> MSGSLSRGNGGKKVLNKNQLLKRNRIRNARSIRAEAVAASSTKTGTPSDLSESGSKLNVDQFISSRQFEVKQLQLAMHNSKAASSTRIFQALPRKLRRRTASHNVRRIPKRMRNRALREMRKSDQQDVLKGSSASSRKAHGLNAKQLYKARMSIKLLRLASKSTSMKLSMPPEVTSSNCHVRQKIKTLKRMIKESSTANPNIKLLNNRMGSYDCTGVNELAPIPKGRVKYTKRQKHFAWLPTHIWNAKRSHMMKRWGYQMVWAPTQKCFKLTHRLGGDTCSSDGALCMDSSYIGTIIVKDKSNDSEGDFLKSIIGKLTAERANLRKYREGQVLFQGLIYSFNEENGEDSTKPLGPCDVFWVQKDTAIIRLHPSIYTQVFNILLQHKEKLTVQDCRYSLASVTLKGAKALESLASCLRSTEYSKSFEQFKMVSMITDHNALPQRCTFAFEAIDPRHLAAPKKLNDSQRKTVNSDDILSLHENYPQDEINAVFNELCDPESRTQSYNNQNTLKEISARRYKLLTATPNSINKTTVPFKESDDPSIPLVIIRRLKTRDWIVVLPWFWLLPLWHLLNRIPRMYHIGLRQFQQIQYENKQLYFPDDYPFTQLGYIENSFYKKEASKTKWDRKPMGKRINFEKIKDIHNTKLPAYSGEIGDFFSSDWRFLQILRNGIDYLQRNDKTLELMDSKKTGQFNAQGVRDINCVNDVLEFCKDYEAKTKAMSLSIEENIPVALCKNRKCQFRTPDSISVNSSSFSLTFFPRCIIAVSCTLLERGHPKDNARIYQVPEKDLEHWLQLAKGVYRPNGRKDHDLKIPLPEVHDLIGFITSGTYHLNCGNGMGIGFIDHHAAIRQPTRYVLIRNVGTNTYRLGEWSKISV;> MSGSLKSLDKKIAKRRQVYKPVLDNPFTNEAHMWPRVHDQPLIWQLLQSSIINKLIHIQSKENYPWELYTDFNEIVQYLSGAHGNSDPVCLFVCNKDPDVPLVLLQQIPLLCYMAPMTVKLVQLPKSAMDTFKSVSKYGMLLLRCDDRVDKKFVSQIQKNVDLLQFPWLNAIKYRPTSVKLLKTTVPIVSKKRQK;> MDRTQTFIKDCLFTKCLEDPEKPFNENRFQDTLLLLPTDGGLTSRLQRQQRKSKLNLDNLQKVSQLESADKQLEKRDYQRINKNSKIALREYINNCKKNTKKCLKLAYENKITDKEDLLHYIEEKHPTIYESLPQYVDFVPMYKELWINYIKELLNITKNLKTFNGSLALLKLSMADYNGALLRVTKSKNKTLIGLQGIVIWDSQKFFIMIVKGNIIDEIKCIPKKGTVFQFEIPISDDDDSALRYSILGDRFKYRSVDRAGRKFKSRRCDDMLYYIQN;> MVRLKSRYILFEIIFPPTDTNVEESVSKADILLSHHRASPADVSIKSILQEIRRSLSLNLGDYGSAKCNSLLQLKYFSNKTSTGIIRCHREDCDLVIMALMLMSKIGDVDGLIVNPVKVSGTIKKIEQFAMRRNSKILNIIKCSQSSHLSDNDFIINDFKKIGRENENENEDD;> MINGVYYNEISRDLDISSSTQCLRFLKETVIPSLANNGNNSTSIQYHGISKNDNIKKSVNKLDKQINMADRSLGLQQVVCIFSYGPHIQKMLSILEIFKKGYIKNNKKIYQWNKLTSFDIKREGRNELQEERLKVPILVTLVSDSEIIDLNLHSFTKQ;> MALKKNTHNKSTKRVTKHPSLKTLTHKQIHTTIFVKSTTPYVSALKRINKFLDSVHKQGSSYVAVLGMGKAVEKTLALGCHFQDQKNKKIEVYTKTIEVLDEVITEGQADIDMESDVEDDDKETQLKKRAVSGVELRIYV;> MGKKTFREWQYFKLSITSFDQDVDDAHAIDQMTWRQWLNNALKRSYGIFGEGVEYSFLHVDDKLAYIRVNHADKDTFSSSISTYISTDELVGSPLTVSILQESSSLRLLEVTDDDRLWLKKVMEEEEQDCKCI;>MLVDLNVPWPQNSYADKVTSQAVNNLIKTLSTLHMLGYTHIAINFTVNHSEKFPNDVKLLNPIDIKRRFGELMDRTGLKLYSRITLIIDDPSKGQSLSKISQAFDIVAALPISEKGLTLSTTNLDIDLLTFQYGSRLPTFLKHKSICSCVNRGVKLEIVYGYALRDVQARRQFVSNVRSVIRSSRSRGIVIGSGAMSPLECRNILGVTSLIKNLGLPSDRCSKAMGDLASLVLLNGRLRNKSHKQTIVTGGGSGNGDDVVNDVQGIDDVQTIKVVKRSMDAEQLGHASKRHKP[2x];> MNKDQAEKYQERSLRQKYNLLHVLPTLNSRALSGLYYKNFHNSVKRYQIMLPEQLKSGKFCSHCGCVYVPNFNASLQLTTNTEQGDSDELGGESMEGPKKCIQVNCLNCEKSKLFEWKSEFVVPTFGQDVSPMINSTSSGKVSYAVKKPQKSKTSTGKERSKKRKLNSLTNLLSKRNQEKKMEKKKSSSLSLESFMK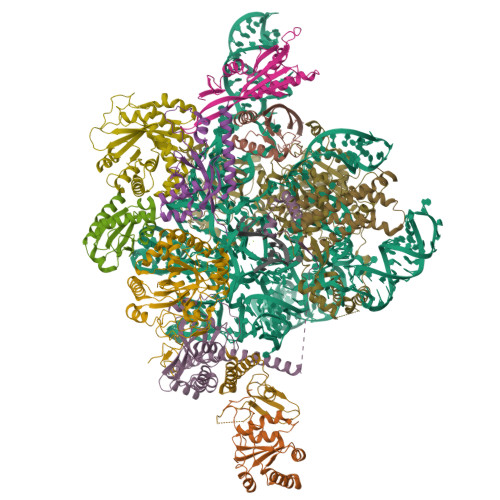S;> MDEMDNVIRSLEQEYRLILLLNHRNKNQHRAASWYGSFNEMKRNCGQIITLFSSRRLQAKRLKDVEWVKLHRLLQRALFRQLKRWYWQFNGVIALGQFVTLGCTLVTLLANVRALYMRLWEINETEFIRCGCLIKNLPRTKAKSVVNDVEELGEIIDEDIGNNVQENELVITSIPKPLTENCKKKKKRKKKNKSAIDGIFG> AFPFF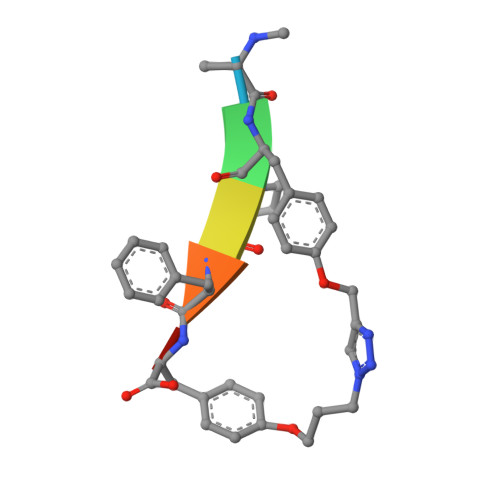X> PADLKDECAQLRRIGDKVNLRQK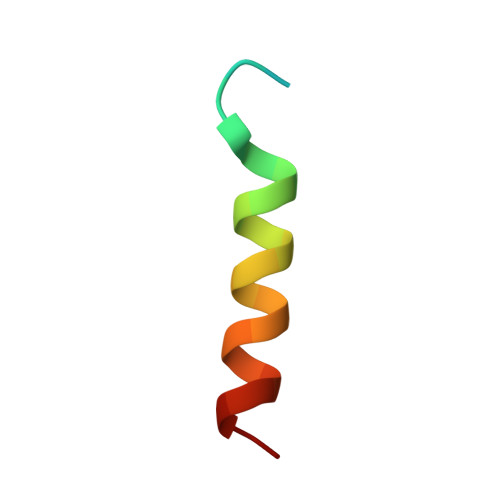LLN>MTITPATHAISINPATGEQLSVLPWAGADDIENALQLAAAGFRDWRETNIDYRAEKLRDIGKALRARSEEMAQMITREMGKPINQARAEVAKSANLCDWYAEHGPAMLKAEPTLVENQQAVIEYRPLGTILAIMPWNFPLWQVMRGAVPIILAGNGYLLKHAPNVMGCAQLIAQVFKDAGIPQGVYGWLNADNDGVSQMIKDSRIAAVTVTGSVRAGAAIGAQAGAALKKCVLELGGSDPFIVLNDADLELAVKAAVAGRYRNTGQVCAAAKRFIIEEGIASAFTERFVAAAAALKMGDPRDEENALGPMARFDLRDELHHQVEKTLAQGARLLLGGEKMAGAGNYYPPTVLANVTPEMTAFREEMFGPVAAITIAKDAEHALELANDSEFGLSATIFTTDETQARQMAARLECGGVFINGYCASDARVAFGGVKKSGFGRELSHFGLHEFCNIQTVWKDRI[4x]

The NAD(P)+-dependent succinate semialdehyde dehydrogenase (SSADH) Sad is a member of the ALDH superfamily and oxidizes succinate semialdehyde (SSA) to succinate. In microorganisms, SSADHs operate in the degradation of various nitrogen-containing compounds such as putrescine or arginine, where they prevent the accumulation of the toxic SSA intermediate. Our results show that Sad is a surprisingly flexible enzyme that is not only able to detoxify succinate semialdehyde and glutarate semialdehyde but can also functionally substitute erythrose 4-phosphate dehydrogenase in pyridoxal 5′-phosphate (PLP) biosynthesis and glyceraldehyde 3-phosphate dehydrogenase (as well as phosphoglycerate kinase) in glycolysis under physiological conditions. We show that Sad, which primarily functions in the detoxification of succinate semialdehyde in various degradation pathways, does not only accept closely related substrates, but also converts phosphorylated sugars as a side reactivity.

EG2.2s had acquired a non-synonymous substitution in sad, resulting in an amino acid change of Q262R; while EG2.3a, EG2.4a, and EG2.5a were predicted by the breseq pipeline28 to carry amplified genomic regions that encoded sad (~80×). To understand the molecular basis of the improved enzyme activity in the Q262R variant, we solved the crystal structures of both Sad WT and Q262R variants with bound NAD+, as well as in complex with both NAD+ and SSA. The Q262R mutation significantly increased activities on E4P and GAP. Further kinetic investigations revealed that the Q262R substitution had significantly improved the Km of Sad for sugar phosphates. While we were not able to obtain structures with sufficient electron densities for the alternative sugar-phosphate substrates, we manually fitted E4P and GAP based on the NAD+/SSA-bound structures. These analyses showed that the Q262R substitution likely altered the electrostatic charge in the active site to better accommodate the carboxyl group of SSA, and/or the phosphate group of E4P and GAP, explaining the dramatically improved kinetic parameters for the E4P dehydrogenase reaction in Sad. R262 is likely responsible for an improved coordination of the phosphate group of E4P and GAP.>[2x]MASEALTMIVNLLRSQRPLQEPTVEQMRAGLEAMAQMSPLPADVELTTVDAGGVPGAWVRVPESDPDRVVLYLHGGGYVIGSIRTHRDLAQRIARAARCRVLLIDYRLAPEHPHPAAVEDSTRAYRWLLETGSDPKRMAIAGDSAGGGLTVATLVALRDAGVPLPAAAVCLSPWVDLEGIGESMTTKAAVDPM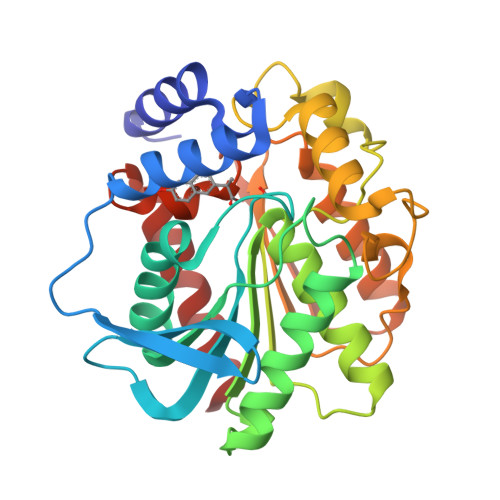VQREPLLRMASMYLAGQDPRTPLAAPLYADLRGLPPLLIQVGTAETLLDDSVRLAERARAAGVQVTLEPWEDMIHVWQAFAAMLPEGQQAIERIGEFLRQHWQ>GKKKRKRCGVCVPCKRLINCGVCSSCRNRKTGHQICKFRKCEE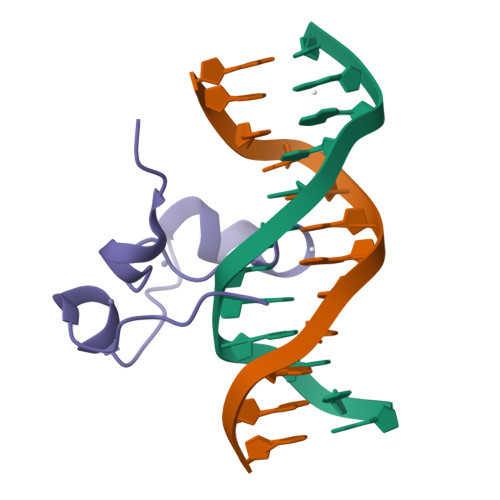LKKKPG[2x]>[2x]ENYARFITAASAARNPSPIRTMTDIL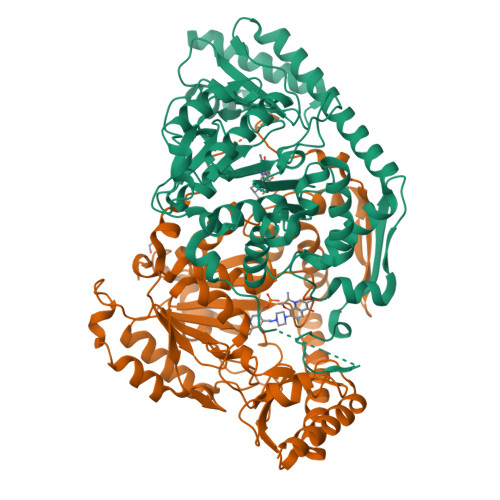SRGPKSMISLAGGLPNPNMFPFKTAVITVENGKTIQFGEEMMKRALQYSPSAGIPELLSWLKQLQIKLHNPPTIHYPPSQGQMDLCVTSGSQQGLCKVFEMIINPGDNVLLDEPAYSGTLQSLHPLGCNIINVASDESGIVPDSLRDILSRWKPEDAKNPQKNTPKFLYTVPNGNNPTGNSLTSERKKEIYELARKYDFLIIEDDPYYFLQFNKFRVPTFLSMDVDGRVIRADSFSKIISSGLRIGFLTGPKPLIERVILHIQVSTLHPSTFNQLMISQLLHEWGEEGFMAHVDRVIDFYSNQKDAILAAADKWLTGLAEWHVPAAGMFLWIKVKGINDVKELIEEKAVKMGVLMLPGNAFYVDSSAPSPYLRASFSSASPEQMDVAFQVLAQLIKESL>[2x]MVAPLLKTLPFLAAAYAAELDLPNFSALNRRQDNSTSSSAGCSLDQTVAPGNLTLCGNATLFTTFRPKARFIAPEGWMNAPMGLYQRADGSIHAGYQSHPKHIQWGNISQGAAYSSDFTSWTDFNGSEGYKTIWPSQIYDIRGVFDGSIIKEGIDGYPTILYTSTSFGPLGATLNEAEGTETQSLAYTTDDGASWIKLGYGAGQNPVIYEWPETNLTGFRDPYVFQSPRLEALLANTTSITNATGDHFATISGGVHGDGARLFLYRQHTTGEFIKWTYLGPLVTTGYKESYGEWSGNYGINFETAGVTRLNPAGAAWDNGSDTTAVDFVTFGTEQGRADHQNHWPLWAAVDYEVRDNGSIEAVIAYSGVQDWGRSYAYASFPVEGYRQVSVGWIYEDDDNVILAKQFGYQGAFTLFRDLFVKVVENVSPSTPGLFEQASWSTKNSTDGMSVTVTTLGQRVVPETLAAYKGNSTVSTLAPVMLNESAAAYTPFSSQPTDRFYALTGSFEFGLNTTAKAGFRVLASEEEYTDIWFDPASENLTVVRTASSLIKSFGNDTELAKVKLYEIVGAESKTLNLTVFVDGSVIEIYANDEVALSTRAYPWLANSTGAGLLADGTTAGDVVGVSGLELWDGLVDAWPARPANTSQGLVWDGPTAAMYGLFAGY

Xanthophyllomyces dendrorhous β-fructofuranosidase (Xd-INV, EC 3.2.1.26) is a highly glycosylated dimeric enzyme that belongs to CAZy family GH32 and hydrolyzes sucrose and various fructooligosaccharides (FOS) and fructans releasing fructose. It also catalyzes the synthesis of short-chain FOS, in which the fructosyl moiety is transferred to the sucrose skeleton. Then, crystals from the inactivated pXd-INV-D80A enzyme were used for soaking experiments into β-D-fructose and the different polyphenols tested, to get the corresponding ternary intermediate complexes. All the polyphenolic compounds are bound by stacking their aromatic rings against Trp105, with additional hydrogen bonds from their OH groups to several residues at the active site directly or through several well-ordered water molecules that are linked to the protein.

For catechol, we detected a small peak in the ELSD chromatogram but it was not appreciable in the UV detector, indicating that the transfructosylation (if it occurs) was not significant. In the ternary complexes with catechol and HQ, a molecule of ethylene glycol from the cryoprotectant solution was also found at the active site. With respect to the crystals containing catechol, the OH linked to the Fru O2 is interacting with the ethylenglycol trapped in the crystals, which in turn is linked to the catalytic Glu303 and to Glu334, through a net of water molecules. The other OH of catechol is linked to a water molecule at the same plane that the aromatic ring, increasing the stacking interface to Trp105. As can be seen, the positions of catechol and the EGCG diphenolic part of benzopirane are very similar, while the aromatic ring of p-nitrophenol is slightly shifted towards the diethylenglycol trapped in the catechol containing crystals. In contrast, catechol/EGCG binding position is shifted from subsite +1 therefore tolerating binding of sucrose donor to a higher extent. In contrast, catechol, HQ, and EGCG bind at the inulin-type subsite +2, occupying the same position that the terminal glucose from 1-kestose. As it is observed, HQ and catechol are similarly located in both ternary complexes, while HQ is shifted in the fructose-free HQ-soaked crystals. A possible explanation is that the higher mobility of HQ allows the second step of the mechanism to proceed, while catechol remains fixed at its position blocking a putative productive motion of the acceptor substrate. Furthermore, the structural superimposition of these complexes with the reported complex of pXd-INV-D80A with sucrose can explain the molecular basis of the partial inhibition observed in sucrose hydrolysis by catechol and EGCG, whose hydrolysis rate is 50–65% referred to the control.> MSQSNRELVVDFLSYKLSQKGYSWSQFMAAVKQALREAGDEFELRYRRAFSDLTSQLHITPGTAYQSFEQVVNELFRDGVNWGRIVAFFSFGGALCV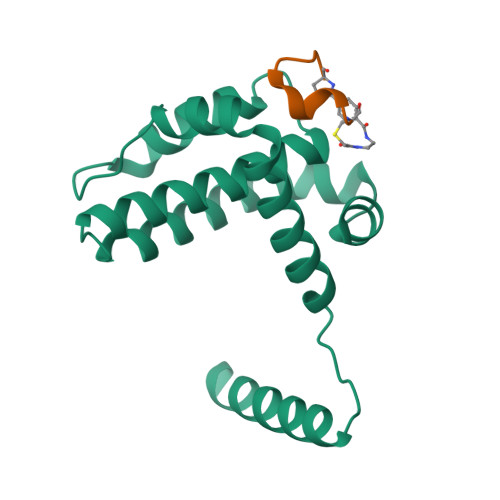ESVDKEMQVLVSRIAAWMATYLNDHLEPWIQENGGWDTFVELYG;> CPARYGWDYECX> MGILFTRIWRLFNHQEHKVIIVGLDNAGKTTILYQFSMNEVVHTSPTIGSNVEEIVINNTRFLMWDIGG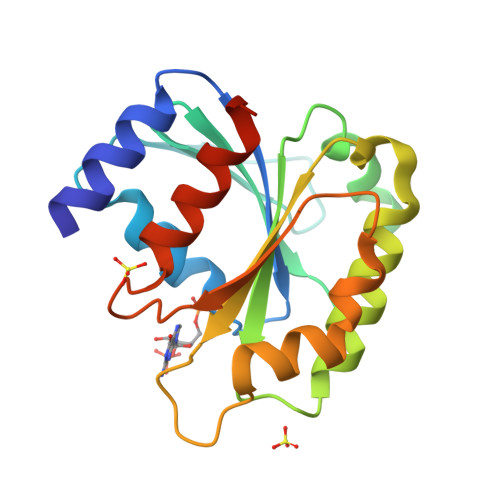QESLRSSWNTYYTNTEFVIVVVDSTDRERISVTREELYKMLAHEDLRKAGLLIFANKQDVKECMTVAEISQFLKLTSIKDHQWHIQACCALTGEGLCQGLEWMMSRLKIRLEHHHHHH Cytoplasmic dynein-1 (dynein) is a highly conserved molecular motor that moves toward the microtubule minus end, transporting various cargoes including RNAs, membrane vesicles, and viruses, and plays a crucial role in cell division. Dynein belongs to the ATPase associated with various cellular activities (AAA+) family of proteins. Its heavy chain features a motor domain composed of six AAA+ modules, a long stalk, a microtubule-binding domain (MTBD) located at the end of the stalk, a buttress region that makes additional connections between the AAA5 module and the stalk, and a long tail that interacts with dynactin and an activating adapter. Lis1 is a dimer (~90 kDa) with an amino-terminal dimerization domain and carboxy-terminal β-propellers that bind to the dynein motor domain24,25. Our data support a model in which Lis1 relieves dynein autoinhibition by increasing its basal ATP hydrolysis rate and promoting conformations compatible with complex assembly and motility.

We also prepared grids with samples that were pre-incubated with Lis1 before ATP addition. Because some of our maps showed partial density for the Lis1 β-propellers, we performed 3D classifications without alignment in Relion to further resolve this compositional heterogeneity. This analysis distinguished states with no, one, or two Lis1 β-propellers bound to dynein. The nucleotide occupancies in these new maps correspond to the nucleotides observed in pre-3D classification maps. In addition, the interaction sites between Lis1 and dynein in our maps are those previously characterized and are largely the same in the bent and intermediate dynein states. We also saw clear density for the second Lis1 β-propeller in the intermediate state dynein, even though the nucleotide densities in this state are consistent with the ones in the straight linker dynein. Comparison of this state (I6, 3.4-Å resolution) with our straight linker dynein (I3, 4-Å resolution) bound to one Lis1 β-propeller showed that the sitering interactions are conserved while sitestalk is shifted away from Lis1 as dynein goes from the intermediate to the straight linker state (~15 Å), making it inaccessible for binding by the second Lis1 β-propeller. Binding of Lis1 at the second site is unlikely to happen without Lis1 bound at sitering. We next investigated the AAA3 and AAA4 contact area and showed that Lis1 binding loosens the AAA3 and AAA4 interface, potentially favoring ADP release from the AAA3 binding pocket. Notably, binding of the second Lis1 β-propeller further loosens the interface, as illustrated by comparing the population distributions of interm-2× Lis1 versus interm-1× Lis1 systems.

> GDQLTHVVEEVKTYDLVWRSIKNLWEDVQRTFETPWCRVDVLLLQSDLANFLRRADELPRAVKQFEMYKSLFSQVNMLTSVNKILVELKDGALKPRHWNMIFRDIGKRQIQKNLLDKLEFSLKDVMVLNLTLNEILLTKIIERAQKEFVIEKSLNRIKKFWKEAQYEVIEHSSGLKLVREWDVLEQACKEDLEELVSMKASNYYKIFEQDCLDLESKLTKLSEIQVNWVEVQFYWLDLYGILGENLDIQNFLPLETSKFKSLTSEYKMITTRAFQLDTTIEVIHIPNFDTTLKLTIDSLKMIKSSLSTFLERQRRQFPRFYFLGNDDLLKIIGSGKHHDQVSKFMKKMFGSIESIIFFEDSITGVRSVEGEVLNLNEKIELKDSIQAQEWLNILDTEIKLSVFTQFRDCLGQLKDGTDIEVVVSKYIFQAILLSAQVMWTELVEKCLQTNEFSKYWKEVDMKIKGLLDKLNKSSDNVKKKIEALLVEYLHFNNVIGQLKNCSTKEEARLLWAKVQKFYQKNDTLDDLNSVFISQSGYLLQYKFEYIGIPERLIYTPLLLVGFATLTDSLHQKYGGCFFGPAGTGKTETVKAFGQNLGRVVVVFNCDDSFDYQVLSRLLVGITQIGAWGCFDEFNRLDEKVLSAVSANIQQIQNGLQVGKSHITLLEEETPLSPHTAVFITLNPGYNGRSELPENLKKSFREFSMKSPQSGTIAEMILQIMGFEDSKSLASKIVHFLELLSSKCSSMNHYHFGLRTLKGVLRNCSPLVSEFGEGEKTVVESLKRVILPSLGDTDELVFKDELSKIFDSAGTPLNSKAIVQCLKDAGQRSGFSMSEEFLKKCMQFYYMQKTQQALILVGKAGCGKTATWKTVIDAMAIFDGHANVVYVIDTKVLTKESLYGSMLKATLEWRDGLFTSILRRVNDDITGTFKNSRIWVVFDSDLDPEYVEAMNSVLDDNKILTLPNGERLPIPPNFRILFETDNLDHTTPATITRCGLLWFSTDVCSISSKIDHLLNKSYEALDNKLSMFELDKLKDLISDSFDMASLTNIFTCSNDLVHILGVRTFNKLETAVQLAVHLISSYRQWFQNLDDKSLKDVITLLIKRSLLYALAGDSTGESQRAFIQTINTYFGHDSQELSDYSTIVIANDKLSFSSFCSEIPSVSLEAHEVMRPDIVIPTIDTIKHEKIFYDLLNSKRGIILCGPPGSGKTMIMNNALRNSSLYDVVGINFSKDTTTEHILSALHRHTNYVTTSKGLTLLPKSDIKNLVLFCDEINLPKLDKYGSQNVVLFLRQLMEKQGFWKTPENKWVTIERIHIVGACNPPTDPGRIPMSERFTRHAAILYLGYPSGKSLSQIYEIYYKAIFKLVPEFRSYTEPFARASVHLYNECKARYSTGLQSHYLFSPRELTRLVRGVYTAINTGPRQTLRSLIRLWAYEAWRIFADRLVGVKEKNSFEQLLYETVDKYLPNQDLGNISSTSLLFSGLLSLDFKEVNKTDLVNFIEERFKTFCDEELEVPMVIHESMVDHILRIDRALKQVQGHMMLIGASRTGKTILTRFVAWLNGLKIVQPKIHRHSNLSDFDMILKKAISDCSLKESRTCLIIDESNILETAFLERMNTLLANADIPDLFQGEEYDKLLNNLRNKTRSLGLLLDTEQELYDWFVGEIAKNLHVVFTICDPTNNKSSAMISSPALFNRCIINWMGDWDTKTMSQVANNMVDVVPMEFTDFIVPEVNKELVFTEPIQTIRDAVVNILIHFDRNFYQKMKVGVNPRSPGYFIDGLRALVKLVTAKYQDLQENQRFVNVGLEKLNESVLKVNELNKTLSKKSTELTEKEKEARSTLDKMLMEQNESERKQEATEEIKKILKVQEEDIRKRKEVVMKSIQDIEPTILEAQRGVKNIKKQQLTEIRSMVNPPSGVKIVMEAVCAILGYQFSNWRDIQQFIRKDDFIHNIVHYDTTLHMKPQIRKYMEEEFLSDPNFTYETINRASKACGPLYQWVNAQINFSKVLENVDPLRQEMKRIEFESLKTKANLLAAEEMTQDLEASIEVSKQKYSLLIRDVEAIKTEMSNVQANLDRSISLVKSLTFEKERWLNTTKQFSKTSQELIGNCIISSIYETYFGHLNERERGDMLVILKRLLGKFAVKYDVNYRFIDYLVTLDEKMKWLECGLDKNDYFLENMSIVMNSQDAVPFLLDPSSHMITVISNYYGNKTVLLSFLEEGFVKRLENAVRFGSVVIIQDGEFFDPIISRLISREFNHAGNRVTVEIGDHEVDVSGDFKLFIHSCDPSGDIPIFLRSRVRLVHFVTNKESIETRIFDITLTEENAEMQRKREDLIKLNTEYRLKLKNLEKRLLEELNNSQGNMLENDELMVTLNNLKKEAMNIEKKLSESEEFFPQFDNLVEEYSIIGKHSVKIFSMLEKFGQFHWFYGISIGQFLSCFKRVFIKKSRETRAARTRVDEILWLLYQEVYCQFSTALDKKFKMIMAMTMFCLYKFDIESEQYKEAVLTMIGVLSESSDGVPKLTVDTNDDLRYLWDYVTTKSYISALNWFKNEFFVDEWNIADVVANSENNYFTMASERDVDGTFKLIELAKASKESLKIIPLGSIENLNYAQEEISKSKIEGGWILLQNIQMSLSWVKTYLHKHVEETKAAEEHEKFKMFMTCHLTGDKLPAPLLQRTDRVVYEDIPGILDTVKDLWGSQFFTGKISGVWSVYCTFLLSWFHALITARTRLVPHGFSKKYYFNDCDFQFASVYLENVLATNSTNNIPWAQVRDHIATIVYGGKIDEEKDLEVVAKLCAHVFCGSDNLQIVPGVRIPQPLLQQSEEEERARLTAILSNTIEPADSLSSWLQLPRESILDYERLQAKEVASSTEQLLQEM;>[2x]GMTNWQQQLPLTDTQKNELDKSVLRYLNWNYKQTVRHEHAQDYESVRHAIVTLSGFLLQESVDRQEFISNNDTSNESMVDIDELLLPKKWNSIVRLQKKIIELEQNTETLVSQIKDLNTQVSELAQFKPTTSNGTSAHNVLKWIPRNLPSCLINVESSVTSVKLHPNLPIVFVATDHGKLYAFDLFNYTIPLASLQSHTKAITSMDVLFTNYTNSSKKNYLVIVTASKDLQIHVFKWVSEECKFQQIRSLLGHEHIVSAVKIWQKNNDVHIASCSRDQTVKIWDFHNGWSLKTFQPHSQWVRSIDVLGDYIISGSHDTTLRLTHWPSGNGLSVGTGHEFPIEKVKFIHFIEDSPEIRFRTPSTDRYKNWGMQYCVSASRDRTIKIWEIPLPTLMAHRAPIPNPTDSNFRCVLTLKGHLSWVRDISIRGQYLFSCADDKSVRCWDLNTGQCLHVWEKLHTGFVNCLDLDVDFDSNVTPRQMMVTGGLDCKSNVFMR> RKLCSLDNGDCDQF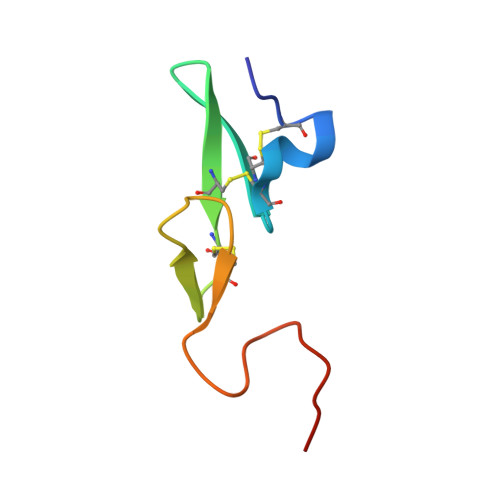CHEEQNSVVCSCARGYTLADNGKACIPTGPYPCGKQTLERR>[4x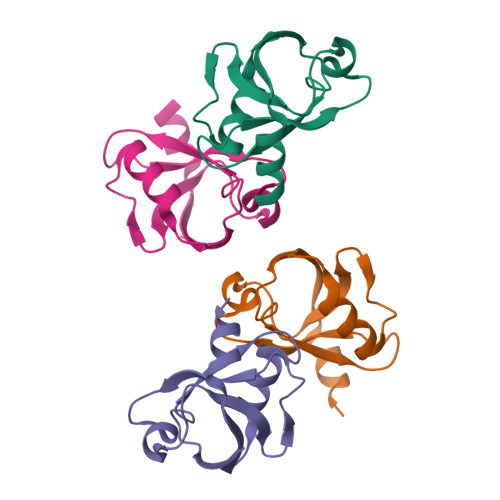]SRRITLNRRPSGLGFNIVGGDNAQGIYVSFISYGGPAEEDGRLQPGDKILQVNSADLSEASHDEAVEIIKKAKSPVNLAVVHDPEGFGRLKSN> GQTVT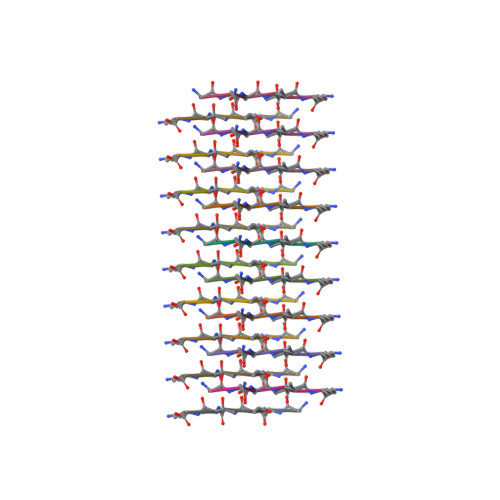K Pseudomonas aeruginosa can also secrete a mART toxin, known as exotoxin A (PE), but with an organization of its three functional domains (receptor, translocation, and enzymatic elements) that is opposite to DT. All these PLTs were composed of a single-chain amino acids that folded into three distinct structures: a receptor binding domain I, a translocation domain II, and a catalytic toxin domain III. Cytotoxicity associated with this family of toxins is due to their enzymatic activity and the ADP-ribosylation of eEF2. Our analysis of four of these new members by X-ray crystallography presents the defining three-domain structure typical of this family, despite substantial variability in the amino acid sequences of these proteins.

We performed a search of public databases using selected hallmarks present in the amino acid sequences of the three known PLTs to identify six additional family members and performed structural and functional assessments of all nine family members. These additional six PLTs were identified across a diverse spectrum of bacterial species: Chromobacterium haemolyticum, Janthinobacterium lividum, Collimonas fungivorans, Serratia fonticola, Acinetobacter baumannii, and Shewanella putrefaciens. Despite having disparate levels of sequence homology, all PLTs had nearly superimposable structures compared to PE with pairwise analysis showing root-mean-square deviation (RMSD) values ranging between 2.3 Å and 3.2 Å (all atoms). Primary sequence alignment of PLT proteins indicates that K57 is conserved in Spx but not in the others. In comparable conditions, Hmx and Jlx appeared to be more readily cleaved by human furin, with Ahx and Spx the slowest, and PE, Chx, Cfx, and Sfx being intermediate at pH 5.5. Variation in the level of cleavage despite strong conservation of the consensus furin-recognition motif and the similar accessibility to this site in all PLT structures suggest that other elements might be at play in mediating the furin-toxin interaction. We superposed the newly identified PLTs with PE and observed extremely high conservation and positioning of residues within the catalytic cleft, indicating that the NAD+ cofactor can be accommodated within this pocket. Remarkably, loops 1 and 2 of all PLTs superpose well with PE, whilst loop 3, which is conserved at the amino acid sequence level, presented more flexibility in our substrate-free structures and may regulate access of the catalytic site to diphthamide. Although we were not able to produce active toxins due to safety concerns, our structural analysis shows that elements involved in NAD+ binding and ADP transferase are conserved in all PLT family members, supporting their putative ADP-ribosylation activity. Only PLT genes in Aeromonas hydrophila, Chromobacterium haemolyticum, Collimonas fungivorans, and Shewanella putrefaciens matched the core gene GC content. Shewanella putrefaciens can infect fish and cause human respiratory and gastrointestinal infections.

>[3x]GVNEAFDLWQECATHCQLDLSQGIRSSELDLTPLFETSNEEGILHYSMLLGEGNEGLKLAIDNALTLHTTHSTINFTSETAESGPRSYSYIRKGENNWSLNWLVPVGDDAPASIKIFFLEQDAVGLNRYISPIYSIEVSNNLLNSLAHKSTFYIRAFDNNQTLSMVNISSAGVSYVAAPQQHHRQKRWSEWHTGKLLCFLDPFDAFYNYVTQHTCNPDDTWEGQIYRVLAGNPATLDTTAPSTTPAVISHRIHFDRGNSLASLTAHQVCGIPLESLARTRHPRGWEELNNCGYPVRNLVSLFILARLSWDRVEQVIHNALTNPTPGNALDDAIREAPERARVTLTLAAAQVNQFDNQAAGNTPEQAQSADVVSLSCSAGALHCSAPADSANALLEREHPNGANFLGAGEAVSFTTRGTRNWSSARLNHAHQQLIARGYVFVGYHGSSLEGAQSIVFGGIRTRTQALDDVWQGLYISGDPAVAYGYAQDQEPDSRGRIRNGTMLRVYVPGTATAYLYETPLTLADPEAVDAVGHLIGHPLPLQTEAITGPEEAGGRPATILGWELAEQAVAIPSTIPTDPSNIGGDLDPSSIPDEESDISALPDNVTKPHHDEL> MFLPPPECPVFEPSWEEFADPFAFIHKIRPIAEQTGICKVRPPPDWQPPFACDVDKLHFTPRIQRLNELEA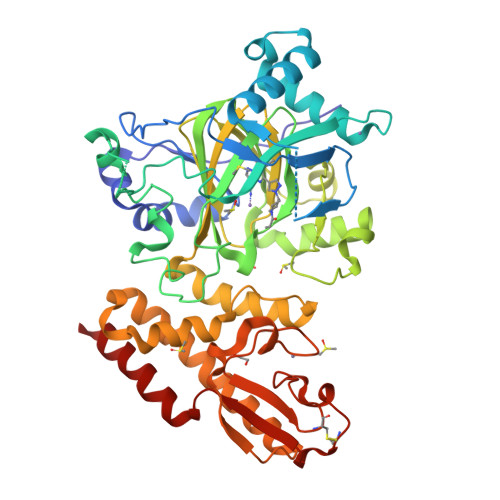QTRGGGGRDYTLRTFGEMADAFKSDYFNMPVHMVPTELVEKEFWRLVSTIEEDVTVEYGADIASKEFGSGFPVRDGKIKLSPEEEEYLDSGWNLNNMPVMEQSVLAHITADICGMKLPWLYVGMCFSSFCWHIEDHWSYSINYLHWGEPKTWYGVPGYAAEQLENVMKKLAPELFVSQPDLLHQLVTIMNPNTLMTHEVPVYRTNQCAGEFVITFPRAYHSGFNQGFNFAEAVNFCTVDWLPLGRQCVEHYRLLHRYCVFSHDEMICKMASKADVLDVVVASTVQKDMAIMIEDEKALRETVRKLGVIDSERMDFELLPDDERQCVKCKTTCFMSAISCSCKPGLLVCLHHVKELCSCPPYKYKLRYRYTLDDLYPMMNALKLRAES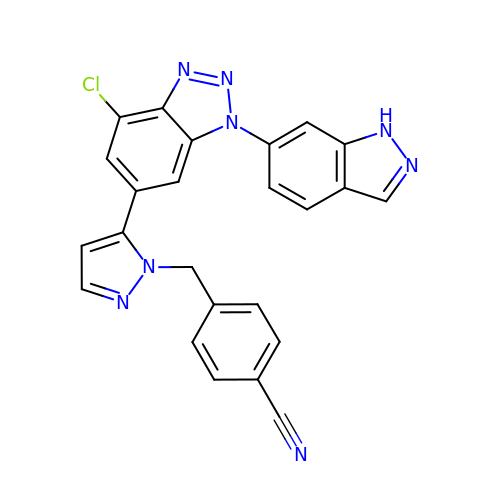4-[[5-[7-chloranyl-3-(1~{H}-indazol-6-yl)benzotriazol-5-yl]pyrazol-1-yl]methyl]benzenecarbonitrile | C24 H15 Cl N8 | WHTYOOSKWPNGMT-UHFFFAOYSA-N> MSGSMEGNAVSFKGGVFS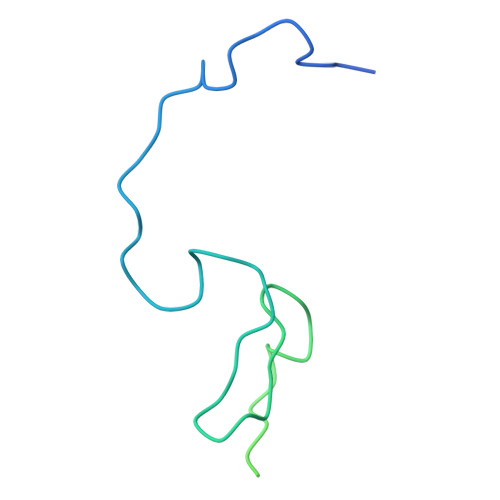PYLTTRLPAWAGVRQNVMGSNVDGRPVAPANSATLTYATVGSSVDTAAAAAASAAASTARGMAADFGLYNQLAASRSLREEDALSVVLTRLEELSQQLQDLFAKVALLNPPANAS> TVENFLGRSACVYMEEYKTTDNDVNKKFVAWPINTKQMVQMRRKLEMFTYLRFDMEVTFVITSRQDPGTTLAQDMPVLTHQIMYVPPGGPIPAKVDDYAWQTSTNPSIFWTEGNAPARMSIPFISIGNAYSNFYDGWSNFDQRGSYGYNTLNNLGHIYVRHVSGSSPHPITSTIRVYFKPKHTRAWVPRPPRLCQYKKAFSVDFTPTPITDTRKDINTVTTV;> GLPTMNTPGSTQFLTSDDFQSPCALPQFDVTPSMNIPGEVKNLMEIAEVDSVVPVNNVQDTTDQMEMFRIPVTINAPLQQQVFGLRLQPGLDSVFKHTLLGEILNYYAHWSGSMKLTFVFCGSAMATGKFLIAYSPPGANPPKTRKDAMLGTHIIWDIGLQSSCVLCVPWISQTHYRLVQQDEYTSAGYVTCWYQTGMIVPPGTPNSSSIMCFASACNDFSVRMLRDTPFISQDNKLQ;> SDRVRSITLGNSTITTQECANVVVGYGRWPTYLRDDEATAEDQPTQPDVATCRFYTLDSIKWEKGSVGWWWKFPEALSDMGLFGQNMQYHYLGRAGYTIHVQCNASKFHQGCLLVVCVPEAEMGGAVVGQAFSATAMANG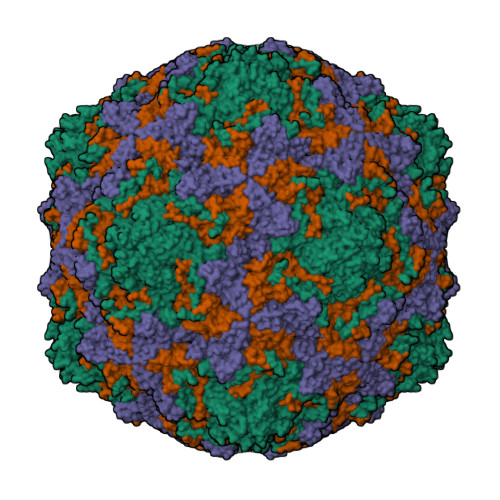DKAYEFTSATQSDQTKVQTAIHNAGMGVGVGNLTIYPHQWINLRTNNSATIVMPYINSVPMDNMFRHYNFTLMVIPFVKLDYADTASTYVPITVTVAPMCAEYNGLRLAQAQ> ALEEIKNGTDISTLDIRKFNLNINNVSVLSKSQSVDQFHLSNPHYEYLSGGAYPGEMENFTLKVDKSKKQDQVFENPLSLKFTNIGTVNGKQVDAYLNFNKVTLHYLNTAQAESEMNSAQKSTVEFFSISELWESNAFEIGNVPYVDANHDYIMNKAFWIDADVTAEIRYADGTETDLKLVMKPTDIDAIDANNLKETFYVKNYQNDVNLRLMNNANVLVQEEASDRTSWIATQITGGSYNENNVSGLALRSNSNSMNFGYSSTETCSAVFGLYIEKIDPRPVLEVDP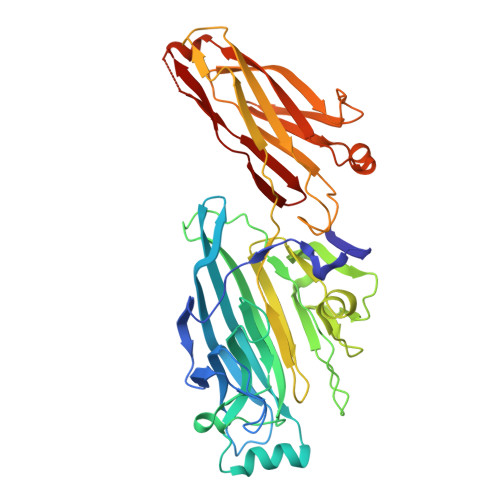AEIPAKDGQDVTYKATFKVPVPGKDILAAPSSIEMVQKFDERLDYKELKVESGGVTLQEGRDYTIEKTGQTVTVKMTPEYLKGNSSSDIIITYKTATNKKVEEKGSEKIDNTVTLHVDNLSAPSNQVSTALLYEK>SRPVRLMKVFVTRRIPAEGRVALARAADCEVEQWDSDEPIPAKELERGVAGAHGLLCLLSDHVDKRILDAAGANLKVISTMSVGIDHLALDEIKKRGIRVGYTPDVLTDTTAELAVSLLLTTCRRLPEAIEEVKNGGWTSWKPLWLCGYGLTQSTVGIIGLGRIGQAI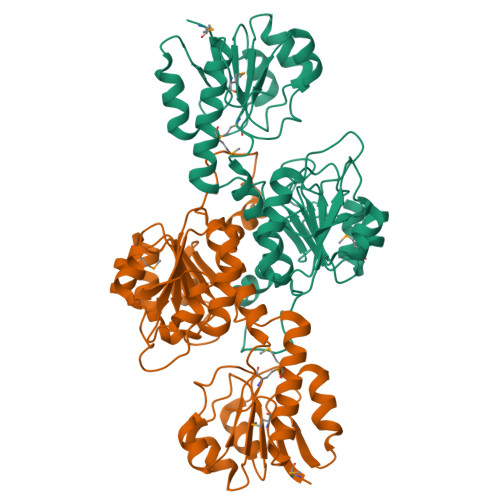ARRLKPFGVQRFLYTGRQPRPEEAAEFQAEFVSTPELAAQSDFIVVACSLTPATEGLCNKDFFQKMKETAVFINISRGDVVNQDDLYQALASGKIAAAGLDVTSPEPLPTNHPLLTLKNCVILPHIGSATHRTRNTMSLLAANNLLAGLRGEPMPSELKL[4x]> GGGGGSP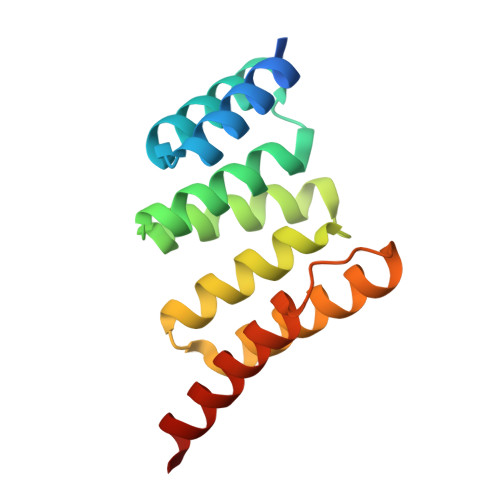EKSPSAQELKEQGNRLFVGRKYPEAAACYGRAITRNPLVAVYYTNRALCYLKMQQHEQALADCRRALELDGQSVKAHFFLGQCQLEMESYDEAIANLQRAYSLAKEQRLNFGDDIPSALRIAKKKRWNSIEER 7-[(3-Chloro-6,7,10,11-tetrahydro-9-methyl-7,11-methanocycloocta[b]quinolin-12-yl)amino]-N-(4-hydroxy-3-methoxybenzyl)heptanamide 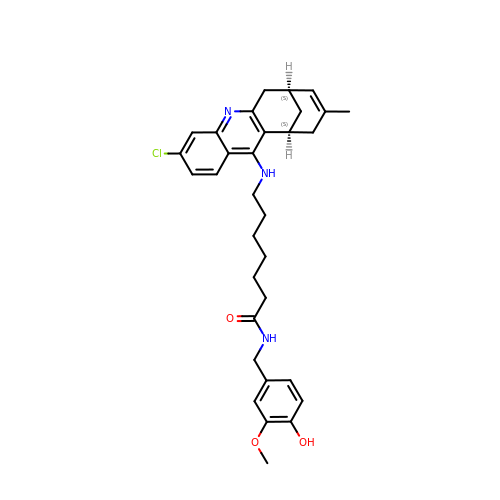| C32 H38 Cl N3 O3 | JGUYMIZRMYBDGV-XZOQPEGZSA-N> XRMKQIEDKIEEIESKQKKIENEIARIKKLLQ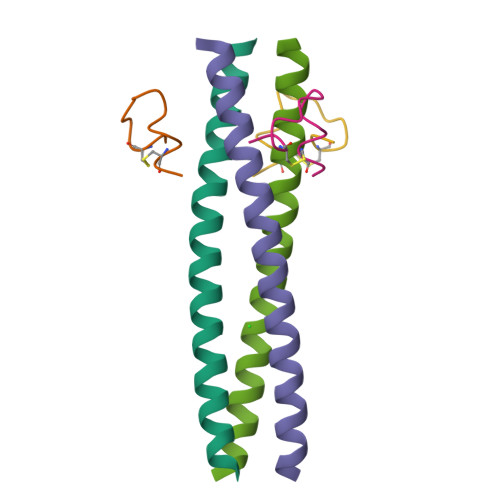LTVWGIKQLQARIL;> XGACEARHREWAWLCAA> GSLHEEADHRVTDHGPRPFVVNIEDETKRNRAFRRALWTGDHLQVTLMSIQVGEDIGLEIHPHLDQFLRVEEGRGLVQMGHRQDNLHFQEEVFDDYAILIPAGTWHNVRNTG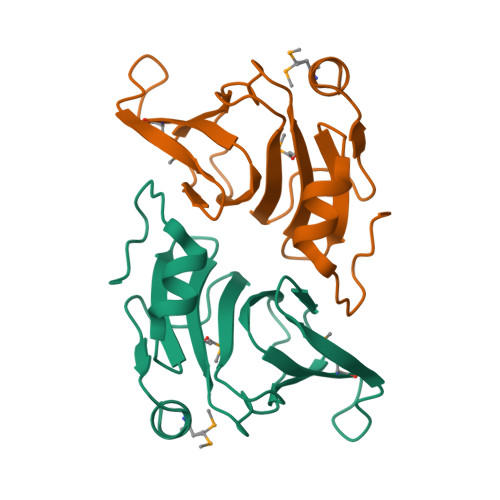NRPLKLYSIYAPPQHPHGTVHETKAIAMAAEEHHHL> LYKKIKDNSILDMRYENNKFIDISGYGSNISINGDVYIYSTNRNQFGIYSSKPSEVNIAQNNDIIYNGRYQNFSISFWVRIPKYFNKVNLNNEYTIIDCIRNNNSGWKISLNYNKIIWTLQDTAGNNQKLVFNYTQMISISDYINKWIFVTITNNRLGNSRIYINGNLIDEKSISNLGDIHVSDNILFKIVGCNDTRYVGIRYFKVFDTELGKTEIETLYSDEPDPSILKDFWGNYLLYNKRYYLLNLLRTDKS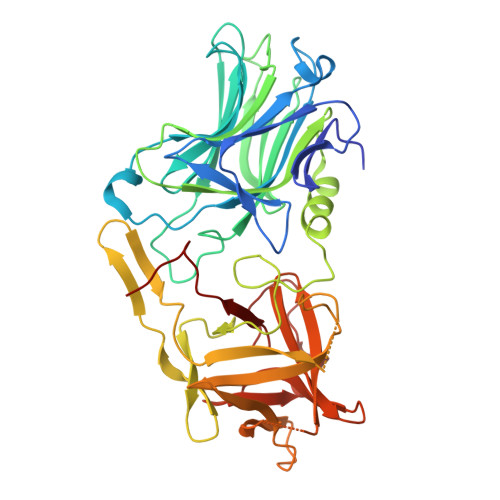ITQNSNFLNINQQRGVYQKPNIFSNTRLYTGVEVIIRKNGSTDISNTDNFVRKNDLAYINVVDRDVEYRLYADISIAKPEKIIKLIRTSNSNNSLGQIIVMDSIGNNCTMNFQNNNGGNIGLLGFHSNNLVASSWYYNNIRKNTSSNGCFWSFISKEHGWQEN>[4x]MKKWIYVVLVLSIAGIGGFSVHAASSAHEKHLNVS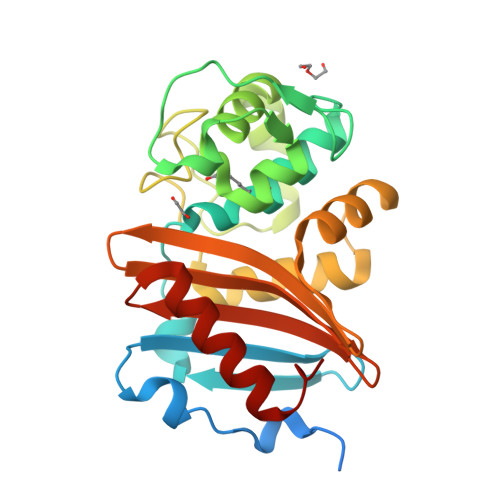KMNVDDEFKDTDGTFILHDLQKDQTFVYNRKRANQRQTPQSTFKVVNALIGLQVKAVRDEYDVKRWDGVKREFESWNRDHTLGSAMRESAIWYYQALARDIGEERMKTWLHTLSYGNEDISGGIDQFWLQSSLTISPLEQETFLEKLAKEELPFDKPVMKIVKRMMIQEEGDHYTLYGKTGTDMGLGWFVGFIKTEHGSYVFVTNVDDSGTKAKNITVDILKKYGLITS>EQLTKCEVFRELKDLKGYGGVSLPEWVCTTFHTSGYDTQAIVQNNDSTEYGLFQINNKIWCKDDQNPHSSNICNI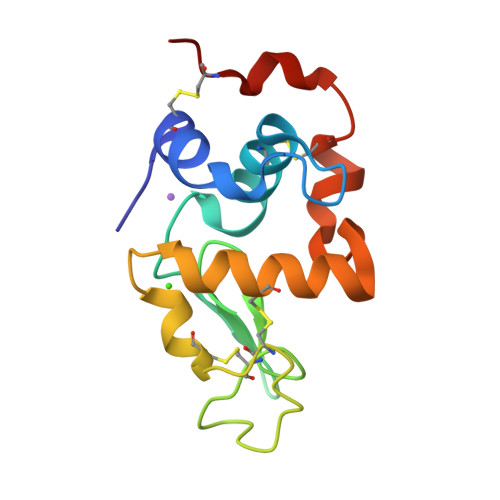SCDKFLDDDLTDDIMCVKKILDKVGINYWLAHKALCSEKLDQWLCEKL[6x]> GSMATVDP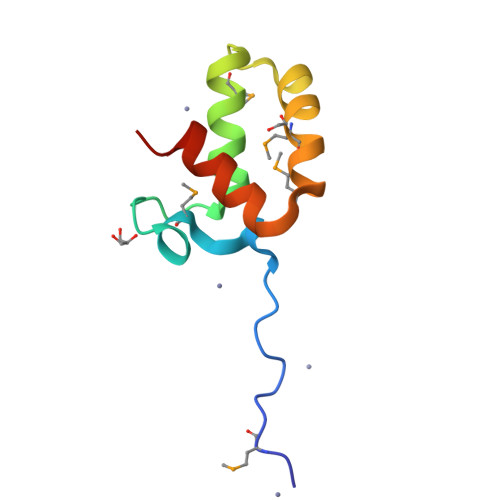EKTLFLDEPMNKVFDWSNSEAPVRDALWDYYMEKNSRDTIKTEEEMKPVLDMSDDEVKALAEKVLKKLE3-(4-bromophenyl)propanal | C9 H9 Br O | 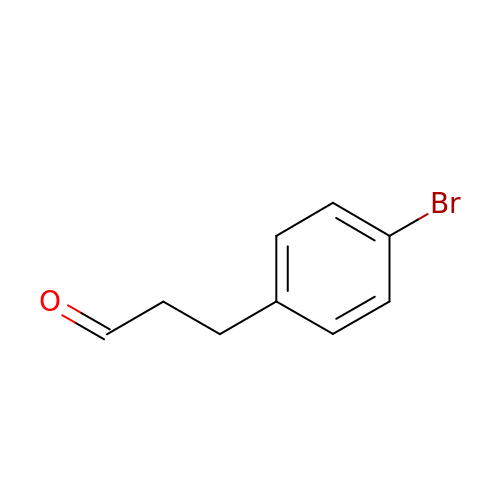RXZJWVPNFPPSEM-UHFFFAOYSA-N>MGHHHHHHMKRKHIKSLIEKIPTAKPELFAYPLDWSIVDSILMERRIRPWINKKIIEYIGEEEATLVDFVCSKVMAHSSPQSILDDVAMVLD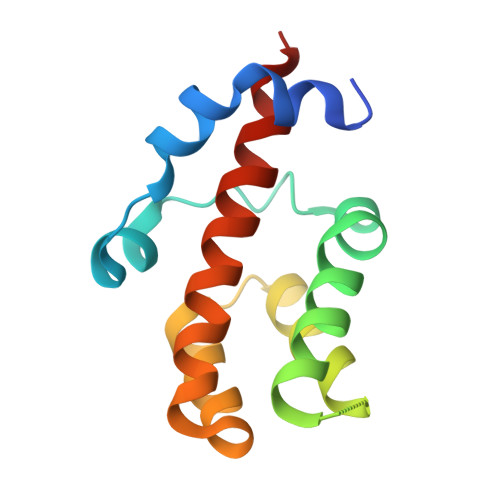EEAEVFIVKMWRLLIYETEAKKIGLVK[5x]> LRITPSRYASKVTAGNAKNQAGSPRQKAKLFHV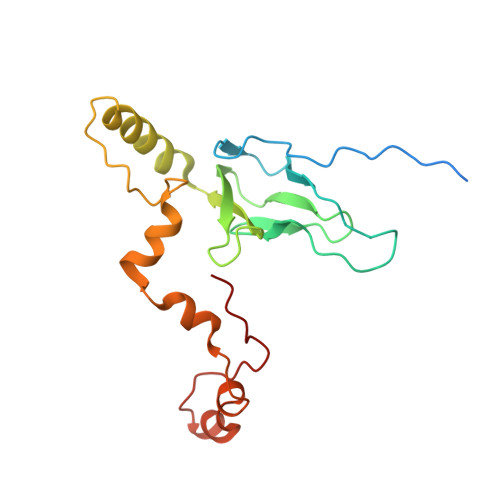IPGTPVTPVEKLKEQRRRFGQDRYSRQPEYRPGRNVRMDPNTFTLYATTKGVMTIRTSRINPSYKWLDVEPDIQKVYRSRCMRAALQARGKASMMVAGNVHYRAELDHVTEPHWRERVMRVPKATERFQDPNYFTRGLVPSLRPLSRYSYE> MRVLATA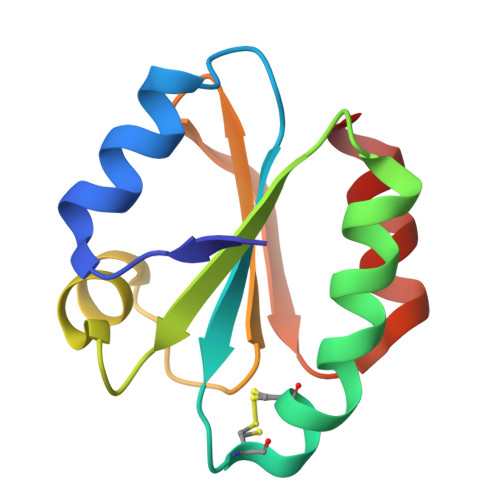ADLEKLINENKGRLIVVDFFAQWCGPCRNIAPKVEALAKEIPEVEFAKVDVDQNEEAAAKYSVTAMPTFVFIKDGKEVDRFSGANETKLRETITRHK>GNYMGNPWTEYMAKYDIEEVHGSGIRVDLGEDAEVAGTQYRLPSGKCPVFGKGIIIENSNTTFLTPVATGNQYLKDGGFAFPPTEPLMSPMTLDEMRHFYKDNKYVKNLDELTLCSRHAGNMIPDNDKNSNYKYPAVYDDKDKKCHILYIAAQENNGPRYCNKDESKRNSMFCFRPAKDISFQNYTYLSKNVVDNWEKVCPRKNLQNAKFGLWVDGNCEDIPHVNEFPAIDLFECNKLVFE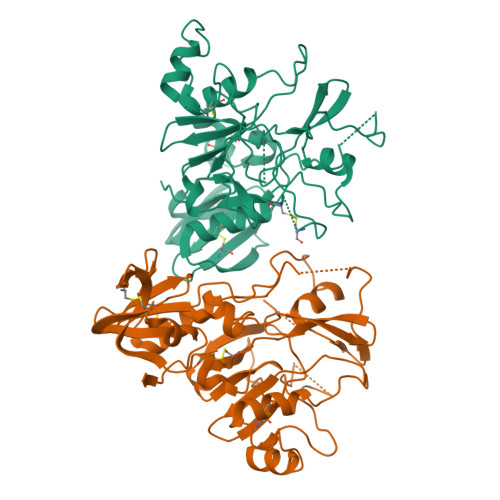LSASDQPKQYEQHLTDYEKIKEGFKNKNASMIKSAFLPTGAFKADRYKSHGKGYNWGNYNTETQKCEIFNVKPTCLINNSSYIATTALSHPIEVE[2x]>[2x]MGHHHHHHYVDRKPSLYLEDLRHDFKNSLSK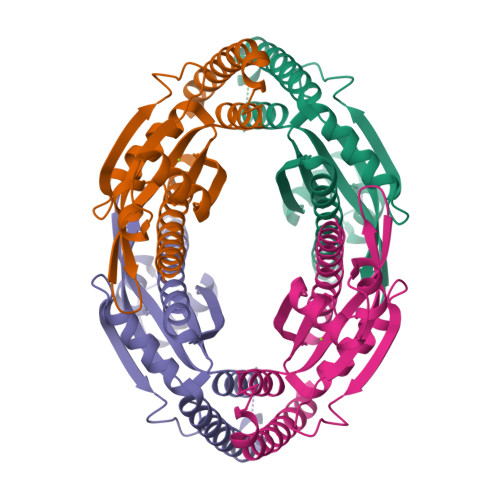FENGDEAFDTLLGFVELDHIYSSALKEISTKLSILDDNFNHIYKHNPIHHMERRVKEMRSLIEKLNRKGLQISAETAKEHILDIAGIRVVCNYLDDIYLIEEMLLKQEDVQLIKRKDYIQHPKENGYRSLHIVVSIPVFLAERVEVLPVEIQIRTIGMDMWASLEHKIRYKNNAETEKYRDLLKECATEITEVEDKLQQIHSEITE> GSIKFTKQSSVASTRNTLKMAQDAERAGMNTLGMLGHQSEQ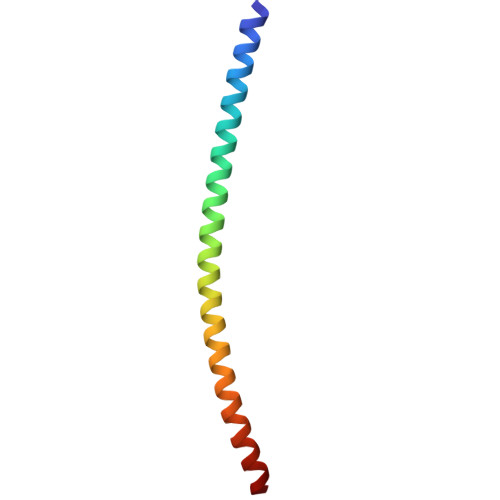LNNVEGNLDLMKVQNKVADEKVAELKKLQ> HHHHHHMRVLGLNGWPRDFHDASAALLVDGRIAAFAEEERFTRKKHGYNTAPVQAAAFCLAQAGLTVDDLDAVAFGWDLPAMYRERLGGWPHSDSEALDILLPRDVFPRRTDPPLHFVQHHLAHAASAYYFSGEDRGAVLIVDGQGEEECVTLAHAEGGKITVLDTVPGAWSLGFFYEHVSEYTGLGGDNPGKLMGLAAHGTTVDETLSAFAFDSDGYRLNLIDPQARDPEDWDEYSVTERAWFAHLERIYRLPPNEFVRRYDPAKGRVVRDTRRDPYEYRDLAATAQAALERAVFGLADSVLARTGERTLFVAGGVGLNATMNGKLLTRSTVDKMFVPPVASDIGVSLGAAAAVAVELGDRIAPMGDTAAWGPEFSPDQVRAALDRTGLAYREPANLEREVAALIASGKVVGWAQGRGEVGPRALGQRSLLGSAHSPTMRDHINLRVADREWWRPFAPSMLRSVSDQVLEVDADFPYMIMTTKVRAAYAERLPSVVHEDWSTRPQTVTEASNPRYHRMLTELGDLVGDPVCLNTSFNDRGEPIVSSPADALLTFSRLPI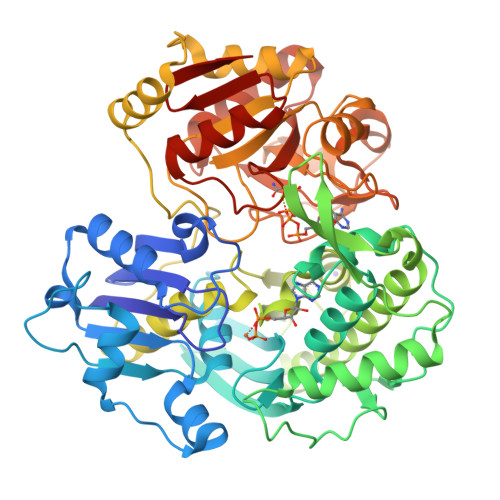DALAVGPYLVTKDLRH>SAEHVLTMLNEHAAAFVRFEATDAAGASRSKSIPAQFFEKVIHARGYLEDGEVNAGAAGAAASDIVLMPELSTAAVAAAAAAATAAVICDGGAAAAASPRYIARAALAQLQAAGAAAGLLSAFIADFCIFGVPEVINSKTISFPASTTAAAADQPQEAAAGGAAGAAAGAAGGAAAAGAAEICFLPEAAGAAAADNAFTLRTGLQEVARRYNAIASAAAAAAAAAAGAGSHSIWDVGAAGTNAFAGASGARATLTGAKWLAGLLAAAAAAAAAAAAAAAAAAAAAAGAAAAAATAWGAAAAACALNIAAAAAAKGAQIENKAGAAAANPYLVLAATVA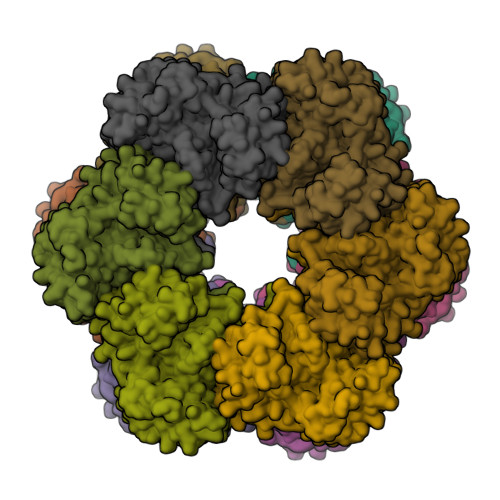AGLDGIQSAGAAAGAAAADAAAAAPSEIPGKMEDALAALEQDAECLKAGLGEAFIRAAVAAAKYELENEETDAEGNKFLEYFI[12x]>MKAVVPTGKIYLGSPFYSDAQRERAAKAKELLAKNPSIAHVFFPFDDGFTDPDEKNPEIGGIRSMVWRDATYQNDLTGI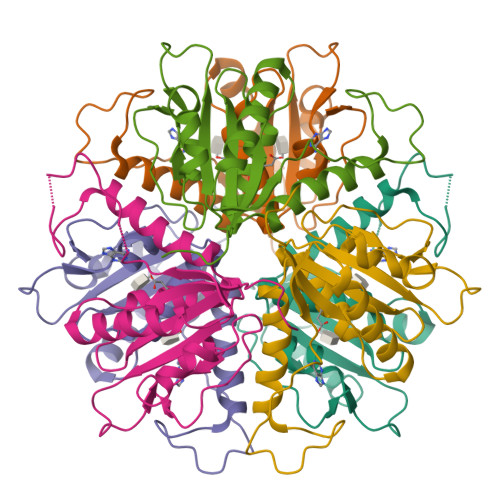SNATCGVFLYDMDQLDDGSAFEIGFMRAMHKPVILVPFTEHPEKEKKMNLMIAQGVTTIIDGNTEFEKLADYNFNECPSNPVRGYGIY[3x]> GPLSFSLGLQDFDLLRVIGRGSYAKVLLVRLKKTDRIYAMKVVKKELVNDDEDIDWVQTEKHVFEQASNHPFLVGLHSCFQTESRLFFVIEYVNGGDLMF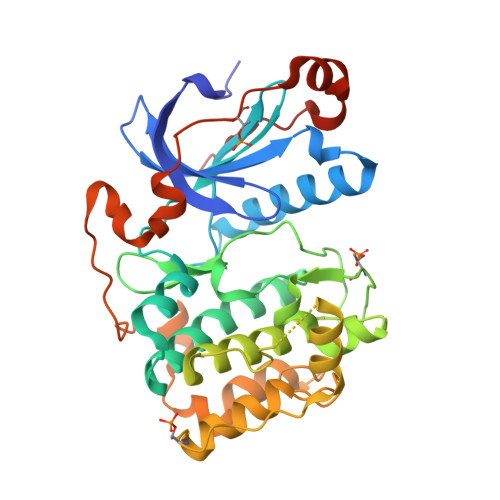HMQRQRKLPEEHARFYSAEISLALNYLHERGIIYRDLKLDNVLLDSEGHIKLTDYGMCKEGLRPGDTTSTFCGTPNYIAPEILRGEDYGFSVDWWALGVLMFEMMAGRSPFDIVGSSDNPDQNTEDYLFQVILEKQIRIPRSLSVKAASVLKSFLNKDPKERLGCHPQTGFADIQGHPFFRNVDWDMMEQKQVVPPFKPNISGEFGLDNFDSQFTNEPVQLTPDDDDIVRKIDQSEFEGFEYINPLLMSAEECV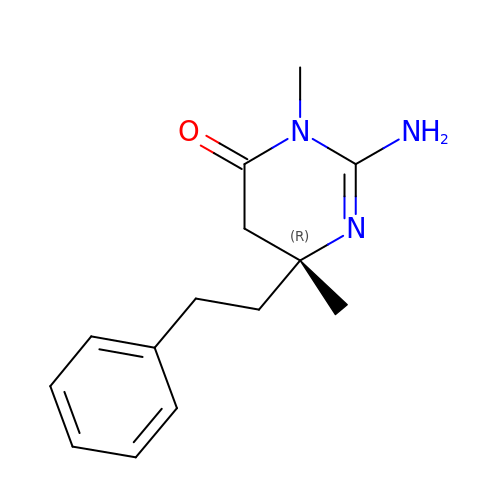(6R)-2-amino-3,6-dimethyl-6-(2-phenylethyl)-5,6-dihydropyrimidin-4(3H)-one | C14 H19 N3 O | NHJCZSSEYRWDOJ-CQSZACIVSA-N Two PGL proteins, PGL-1 and PGL-3, are key scaffolding proteins required for proper P granule assembly. PGL proteins can self-assemble into granules, both in vitro using purified recombinant protein9,11,12 and in intestinal nematode cells or mammalian cells in culture when expressed on their own. These in vitro PGL granules display liquid droplet behavior, indicating that PGL protein alone is sufficient to recapitulate the biophysical properties of P granules in nematode cells. Assays for granule assembly in mammalian cells implicated the conserved N-terminal region of PGL as critical, and structural studies identified a central dimerization domain (DD) within that conserved region.

We determined the Caenorhabditis japonica PGL-1 NtDD crystal structure to 1.5 Å. The NtDD has a novel fold consisting of 11 alpha helices and a single N-terminal beta strand. The asymmetric unit (ASU) was composed of four NtDD domains, which were structurally similar (RMSD 0.219–0.254, C-alpha chains B-D aligned to C-alpha A) except amino acid G114, and the first three N-terminal residues could not be visualized in all of the copies of the ASU. While each ASU possessed two pairs of identical interfaces, one of these interface pairs consisted of a network of conserved amino acid side chains making extensive salt bridges and hydrogen bonds. The complexity and conservation of these interactions suggested biological relevance. Recombinant PGL-1 and PGL-3 NtDD each dimerized on a sizing column combined with multi-angle light scattering (SEC-MALS). PGL-1 and PGL-3 NtDD interface mutants formed monomers rather than dimers in solution. We conclude that the dimers observed in the crystal structure represent the NtDD dimer detected in solution. Therefore, PGL proteins possess two dimerization domains. Based on insights from the NtDD structure, we designed two distinct PGL-1 mutant proteins that are unable to dimerize in vitro and are severely compromised in vivo for assembly into P granules and fertility.

>MDTNKREIVEFLGIRTYFFPNLALYAVNNDELLVSDPNKANSFAAYVFGASDKKPSVDDIVQILFPSGSDSGTILTSMDTLLALGPDFLTEFKKRNQDLARFNLTHDLSILAQGDEDAAKKKLNLMGRKAKLQKTEAAKILAILIKTINSEENYEKFTELSELCGLDLDFDAYVFTKILGLEDEDTADEVEVIRDNFLNRLDQTKPKLADIIRNGP[4x]>[48x]MAAVINTNYLSLVAQNNLNKSQSSLGTAIERLSSGLRINSAKDDAAGMAIANRFTANVRGLTQAARNANDGISLAQTTEGAASEVNTHLQRIRELTVQASNGSYSQEQLDSVQGEINQRLADIDRISEQTDFNGVKVLSDSAKPLTLQVGANDGETITLNLSEISVKTLGLDGFNVNGKGVTQNRSATVTDVIAQGGTLQGDGTYKATTTFNAASAETVLSKLEDGNTVAVGGGATYTYDAAKGNFTYTKTVDTTVGADVTALAN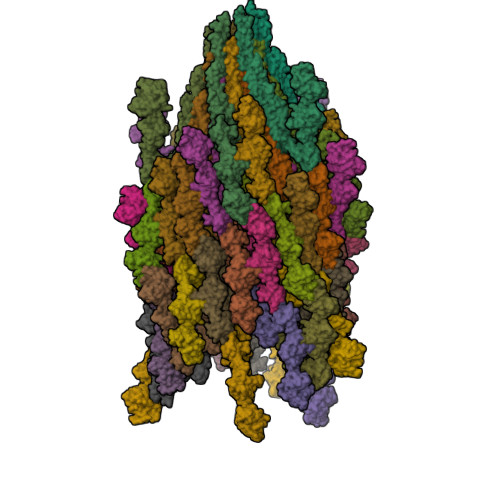KIKPSSGTISGSYEISTGKSASFDVDAAGKITIGGNAAFLNADGELTTNDASGALTQATLDDVLTSVGTEANSSVTIGGTKYSHSAADELSYTAVATTADVLSAMGSSTAVSTVTLGSGITSAAVTFAIATTDSNNTWVDNKGELTDIQTFDTSYKINADTGEVTVVGDNSATAGQYASADGAKVLVGSDGKLTTETTSAGDKTTDPLKTLDAAFTKLDKLTGELGAVQNRLESTIANLNNVVNNLSSARSRIQDADYATEVSNMSKAQILQQAGTSVLAQANQVPQTVLSLLR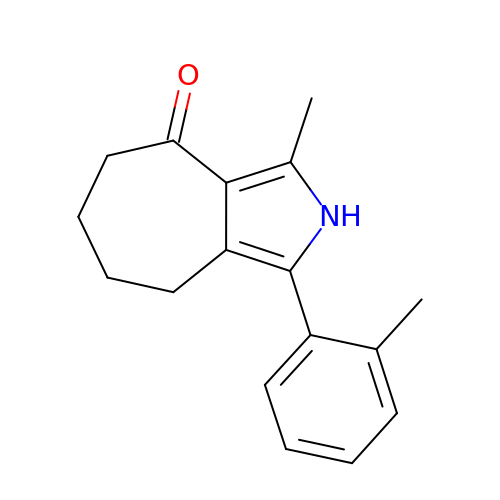3-methyl-1-(2-methylphenyl)-5,6,7,8-tetrahydro-2~{H}-cyclohepta[c]pyrrol-4-one | C17 H19 N O | IZDRTTVDHAXLMR-UHFFFAOYSA-N> GSATIDMNFQSDLLSIF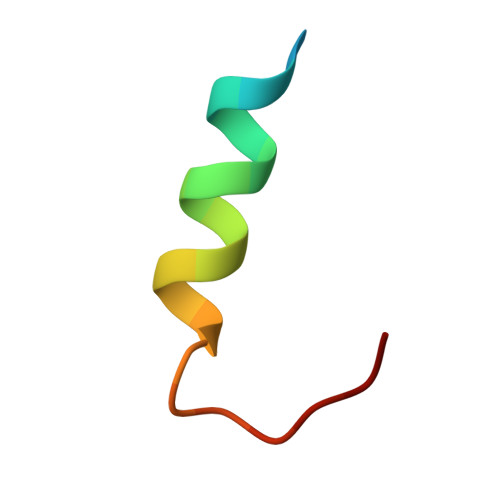EENLF>[4x]PTMTARQRVWRAFENPHTSTMALVFYYVTGFFIAVSVIANVVETVPCGSSPGHIKELPCGERYAV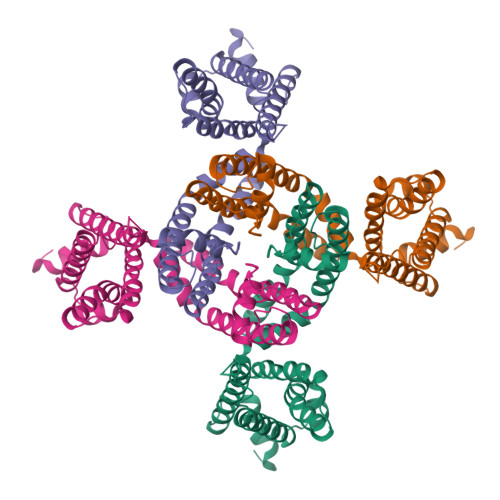AFFCLDTACVMIFTVEYLLRLAAAPSRYRFVRSVMSIIDVVAILPYYIGLVMTDNEDVSGAFVTLRVFRVFRIFKFSRHSQGLRILGYTLKSCASELGFLLFSLTMAIIIFATVMFYAEKGSSASKFTSIPAAFWYTIVTMTTLGYGDMVPKTIAGKIFGSICSLSGVLVIALPVPVIVSNFSRIYHQNQ> METKWLLSKVPDDKSRFEIELEFV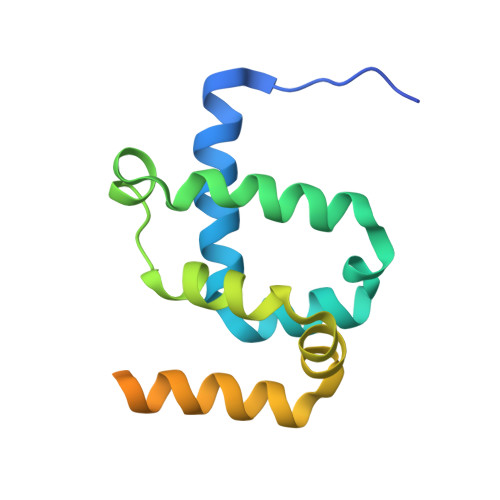QMLSNPWYLNFLAQHKYFEDEAFLQYLEYMEYWREPEYVKFIIYPTCLHMLTLLKNPQFRNDISRADLSKQVNDEIYYEWLGKGLQQYGSADDATLSQPQQEEDEKKVDVKKENE> MQNPTQTMHIYDMPLRV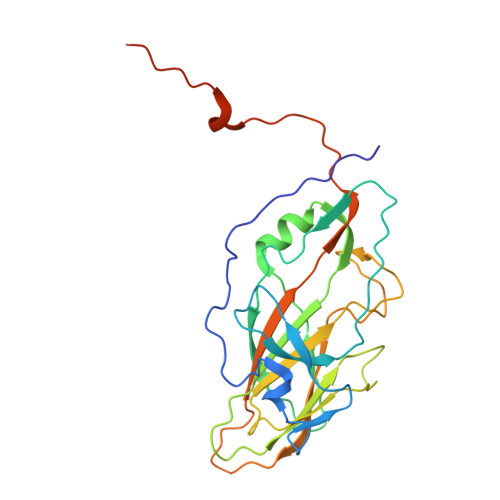IAGLSTLAKTTEEDDNTSTGIVVSEVGEPQVVNHPAWIDPFVAYQLRAPRKNITPDFIFGRADIGNAFSAFLPRRFSAPAVGTRLVVDPVFTYQQRTVLGLYNYFHADFYYIVHVPAPLGTGIYLKIYAPEFDTTTVTRGIRFKPSASPTIALSVPWSNDLSTVETSVGRVGQSGGSIVIETIEDNSNETVNTPLSITVWCCMANIKATGYRHADTSAYNEKGMNFIPVPVPKPPVPPTKPITGEEQ~{N},2,4,6-tetramethylbenzenesulfonamide | C10 H15 N O2 S 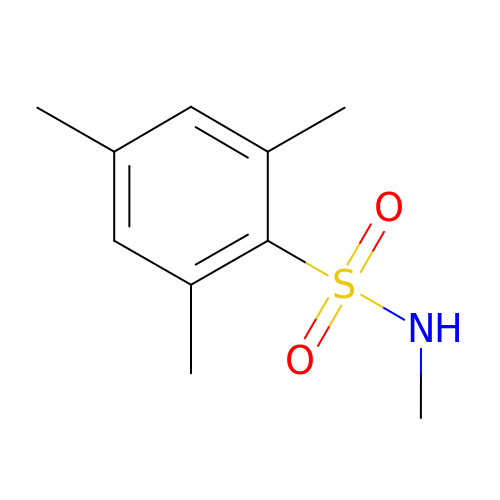| MIMYTDNFDINXHB-UHFFFAOYSA-N>SMTVCQLYAKQIRHRGNVKHNTKLGRERLMRILEQDRLGSCPIDSVKLSDAKEWALRMKEKGLSYKTINND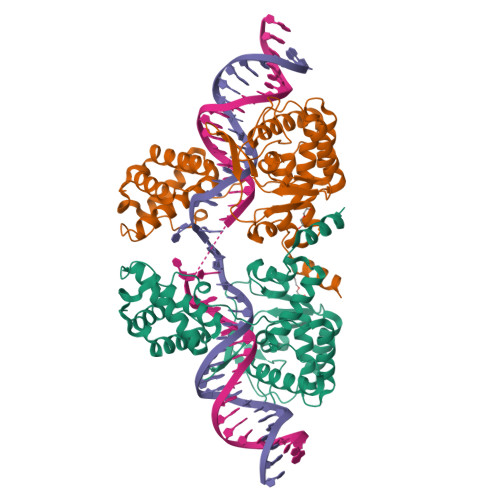KRSLKAAFYTAIQDDCIRKNPFDFQLSDVLDDDTEPKVPLTPAQEESFLSFIQGDKVYQKHYDAIVILLGTGLKISELCGLTDKDLDFENRVIIVSHQLLRNTGVGYYIDEPKTQSGVRKIPMNEEVYQAFQRVIKNRKGAKPFIIDGYANFLFLKQNGYPMTAVDYGGMFGRLVKKYNKSHEEALPKTTTPHAMRHTFCTRLANAGMNPKALQYIMGHSNITMTLNYYAHATFDSARAEMERLAA[2x]(2R)-1-(dodecanoyloxy)-3-hydroxypropan-2-yl (5E,8E,11E)-tetradeca-5,8,11-trienoate 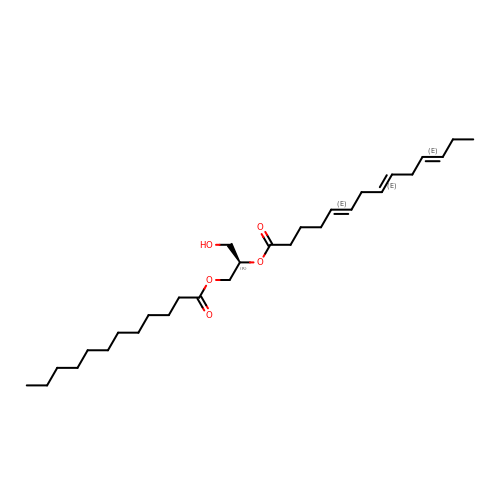| C29 H50 O5 | VISPTZOKUBCLGQ-AUBZEWDZSA-N>[2x]MQQKAQITSQQLRKAQLQVDRFAMELEQSRNLSNTIVHIDMDAFYAAVEM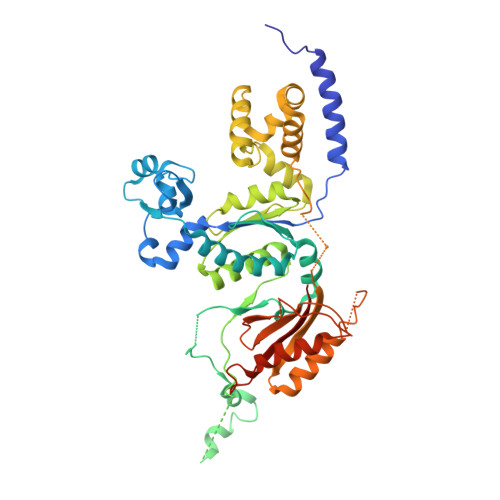RDNPELKDKPIAVGSMSMLSTSNYHARRFGVRAAMPGFIAKRLCPQLIIVPPNFDKYRAVSKEVKEILADYDPNFMAMSLDEAYLNITKHLEERQNWPEDKRRYFIKMGSSVENDNPGKEVNKLSEHERSISPLLFEESPSDVQPPGDPFQVNFEEQNNPQILQNSVVFGTSAQEVVKEIRFRIEQKTTLTASAGIAPNTMLAKVCSDKNKPNGQYQILPNRQAVMDFIKDLPIRKVSGIGKVTEKMLKALGIITCTELYQQRALLSLLFSETSWHYFLHISLGLGSTHLTRDGERKSMSVERTFSEINKAEEQYSLCQELCSELAQDLQKERLKGRTVTIKLKNVNFEVKTRASTVSSVVSTAEEIFAIAKELLKTEIDADFPHPLRLRLMGVRISSFPNEEDRKHQQ>GSHMAAELDSLLGQEKERFQVLPGRDKMLYVAAQNERDTLWARQVLARGDYDKNARVINENEENKRISIWLDTYYPQLAYYRIHFDEPRKPVFWLSRQRNTMSKKELEVLSQKLRALMPYADSVNITLMDDVTAAGQAEAGLKQQALPYSRRNHKGGVTFVIQGALDDVEILRARQFVDSYYRTWGGRYVQFAIELKDDWLKGRSFQYGAEGYI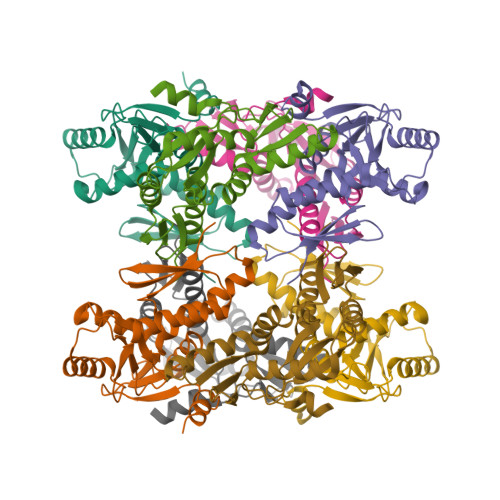KMSPGHWYFPSPL[8x]> FQGAMSSSIDISKINSWNKEFQSDLTHQLATTVLKNYNADDALLNKTRLQKQDNRVFNTVVSTDSTPVTNQKSSGRCWLFAATNQLRLNVLSELNLKEFELSQAYLFFYDKLEKANYFLDQIVSSADQDIDSRLVQYLLAAPTEDGGQYSMFLNLVKKYG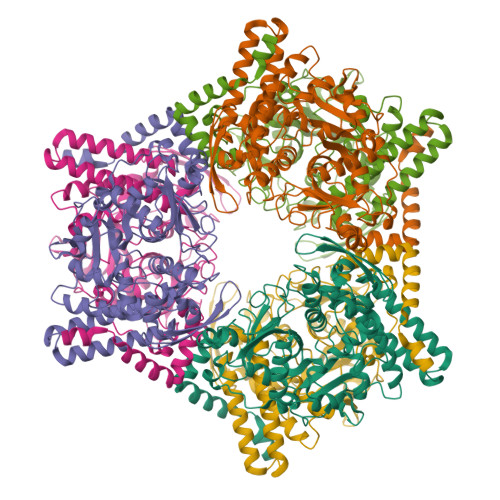LIPKDLYGDLPYSTTASRKWNSLLTTKLREFAETLRTALKERSADDSIIVTLREQMQREIFRLMSLFMDIPPVQPNEQFTWEYVDKDKKIHTIKSTPLEFASKYAKLDPSTPVSLINDPRHPYGKLIKIDRLGNVLGGDAVIYLNVDNETLSKLVVKRLQNNKAVFFGSHTPKFMDKKTGVMDIELWNYPAIGYNLPQQKASRIRYHESLMTHAMLITGCHVDETSKLPLRYRVELSWGKDSGKDGLYVMTQKYFEEYCFQIVVDINELPKELASKFTSGKEEPIVLPIWDPMGALA>[2x]MSLAKISKIEAQKRKGRYNIYLDGKYAFPVAESVLIQ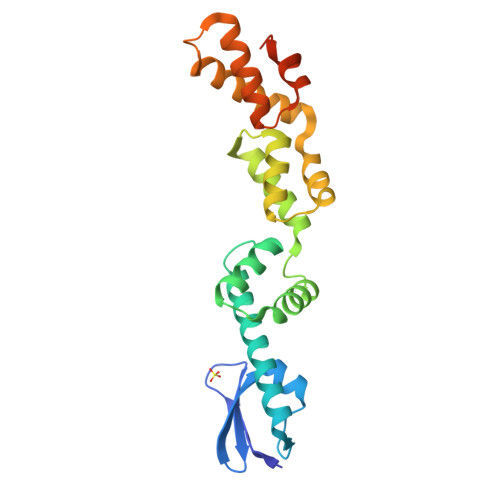FRLMKGTELDEKQIAAIATADQQAKAYSRMLDYLSYQMRTESDIVKKLKEIDTPEEFVEPILKKLRGQQLIDDHAYAASYVRTMINTDLKGPGIIRQHLRQKGIGESDIDDALTQFTPEVQAELAKKLALKLFRRYRNQPERRREQKVQQGLTTKGFSSSVYEMIKDEVVPQPDLEEGHHHHHH> GHMKIKIVPAVGGGSPLELEVAPNATVGAVRTKVCAMKKLPPDTTRLTY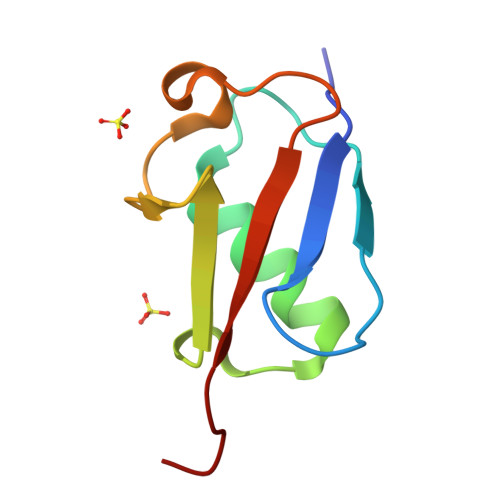KGRALKDTETLESLGVADGDKFVLITRTVGG> SNAATSTVKQEITEGINRYLYSIDKADPTLGKQLFYVSPETSFIHPRGH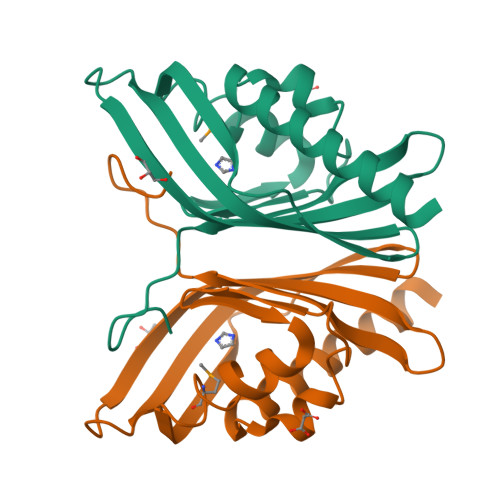ERGWSQIAENFYGTTMGKTFSKRTLKLDAPPAIHVYGNAAVAEFDWHFTAVRRDNGQTQHTTGRESQVWAKIPNTGWRIVHVHYSGPAKTGVGEGY>[2x]NKYNSEILNNIILNLRYKDNNLIDLSGYGAKVEVYDGVELNDKNQFKLTSSANSKIRVTQNQNIIFNSVFLDFSVSFWIRIPKYKNDGIQNYIHNEYTIINCMKNNSGWKISIRGNRIIWTLIDINGKTKSVFFEYNIREDISEYINRWFFVTITNNLNNAKIYINGKLESNTDIKDIREVIANGEIIFKLDGDIDRTQFIWMKYFSIF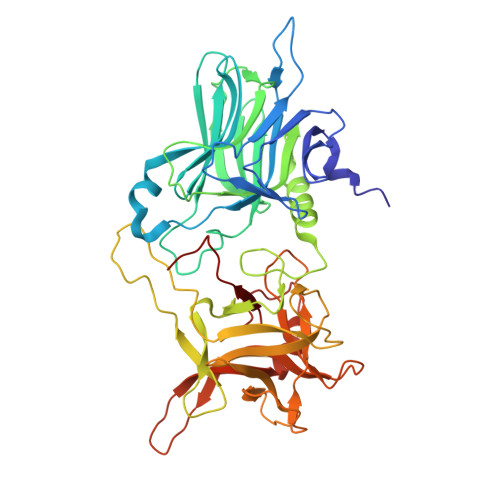NTELSQSNIEERYKIQSYSEYLKDFWGNPLMYNKEYYMFNAGNKNSYIKLKKDSPVGEILTRSKYNQNSKYINYRDLYIGEKFIIRRKSNSQSINDDIVRKEDYIYLDFFNLNQEWRVYTYKYFKKEEEKLFLAPISDSDEFYNTIQIKEYDEQPTYSCQLLFKKDEESTDEIGLIGIHRFYESGIVFEEYKDYFCISKWYLKEVKRKPYNLKLGCNWQFIPKDEGWTE> MEHVAFGSEDIENTLAKMDDGQLDGLAFGAIQLDGDGNILQYNAAEGDITGRDPKQVIGKNFFKDVAPCTDSPEFYGKFKEGVASGNLNTMFEYTFDQQMTPTKVKV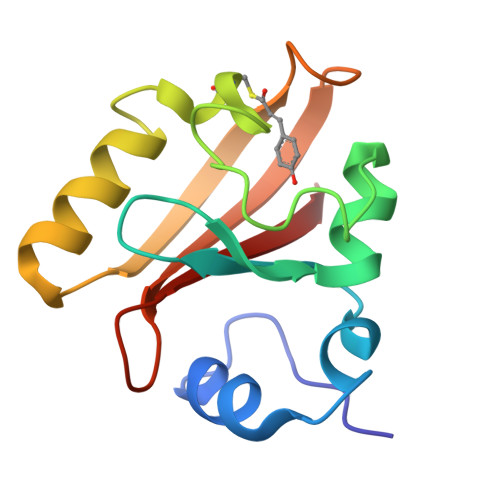HMKKALSGDSYWVFVKRV>GCAGUG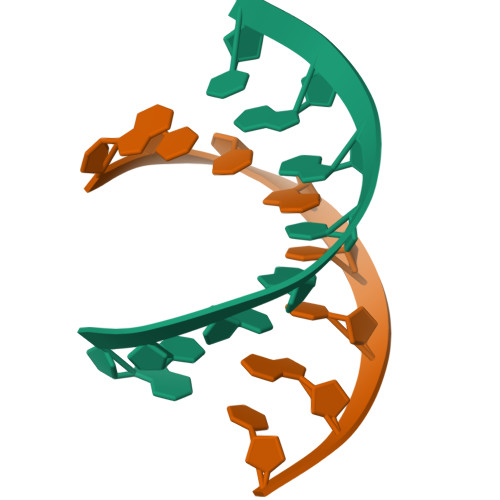GC[2x];>[2x]GCCACTGC> EAYTLSTLAALPAAEIVRLANSQSSSGLPLPKADPATVKATDDFIDSLQGKAAHDQKQKLGDQLFK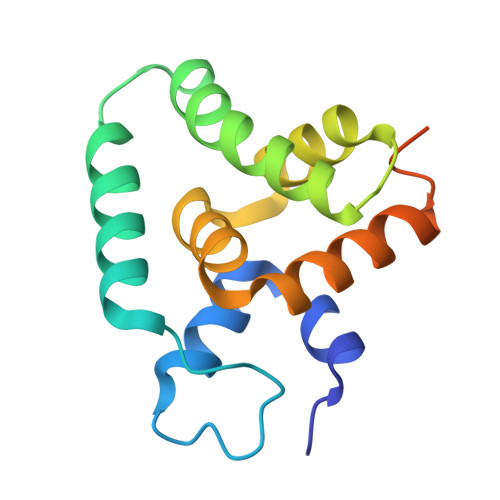KIRTFGVKGAPKLTIHLLDSEDLRALAHLMNSYEDVLKEKVQHKVAAGLNKFGVKGAPKLTIHLLDSED Nicotinamide phosphoribosyltransferase (NAMPT) plays an important role in the biosynthesis of nicotinamide adenine dinucleotide (NAD+) via the nicotinamide (NAM) salvage pathway. Here, we demonstrated the NAMPT-mediated salvage pathway is functional in the Gram-negative phytopathogenic bacterium Xanthomonas campestris pv. campestris (Xcc) for the synthesis of NAD+, and the enzyme activity of NAMPT in this bacterium is significantly higher than that of human NAMPT in vitro. Our structural analyses of Xcc NAMPT, both in isolation and in complex with either the substrate NAM or the product nicotinamide mononucleotide (NMN), uncovered significant details of substrate recognition. Specifically, we revealed the presence of a NAM binding tunnel that connects the active site, and this tunnel is essential for both catalysis and inhibitor binding.

To gain insights into the functional significance of the tunnel in NAMPT catalysis, we introduced mutations to amino acids within the internal cavity of the tunnel and investigated their impact on enzyme activity. To completely block the tunnel, which had a large diameter, we made multiple substitutions using bulky aromatic residues simultaneously. This led to the creation of the H175F-I224F-V291F-I332F mutant, where four residues were each replaced by a phenylalanine. The crystal structure of this quadruple mutant was determined (3.11 Å), which confirmed that the tunnel had been successfully blocked. By comparing the structure of the mutant with that of the NAMPT-NAM complex, we discovered that the presence of the aromatic side chain of Phe 224 caused a conflict with the NAM molecule bound within the tunnel. Consequently, the binding of NAM to this site would be either significantly reduced or completely lost in the mutant. Specifically, blocking the tunnel caused a 129-fold increase in Km and a 3.35-fold decrease in kcat for the substrate NAM, resulting in a 403-fold decrease in catalytic efficiency. Consistent with the positively cooperative model and the existence of two NAM binding sites, the hill coefficient of the quadruple mutant dropped to 1.00, indicating a loss of positive cooperativity after blocking the tunnel. Our ITC results also supported these findings, as the affinity between the quadruple mutant and NAM was undetectable, indicating a significant reduction in NAM binding at the catalytic site without binding at the tunnel location. However, the quadruple mutant with blocked tunnel was significantly less sensitive to FK866 inhibition, exhibiting an IC50 value of 153.54 nM, which is more than 600-fold higher than that of the wild-type enzyme.

>[2x]MGSSHHHHHHSQGSMHYLDNLLLNTDSYKASHWLQYPPGTDASFFYVESRGGVYDQTAFFGLQSILKEAINRPVTHADIDDAKALLAAHGEPFNEAGWRDIVDRLGGQLPIRIRAVPEGCVVPTHNVLMTIESTDAKAFWVPSYLETLLLRVWYPVTVATVSWQVKQIVRDFLQRTSDDPEGQLPFKLFDFGARGVSSLGSAALGGAAHLVNFLGTDTLSALLLARAHYHTPVAGYSFPAAEHSTITSWGREREVDAYRNMLTQFARPGAIVAVVSDSYDIYRAIREHWGTTLREEIIASGATVFIRPDSGDPVDVVEQCLLLLDEAFGHQVNGKGYKVLNHVRVFQGDGINPQSLRAILERITAAGYAADNVAFGMGGALLQKVDRDTQKFALKCSAVRVDGAWIDVYKDPITDQGKQSKRGRLTLLRDRATGQYRSALLDEVATHAGDSDDALVTVWENGQMLREWTLEQVRAHADAARL>SMTIRSYKNLNLVRANIETESRQFIENKNYSIQSIGPMPGSRAGLRVVFTRPGVNLATVDIFYNGDGSTTIQYLTGANRSLGQELADHLFETINPAEFEQVNMVLQGFVETSVLPVLELSADESHIEFREHSRNAHTVVWKIISTSYQDELTVSLHITTGKLQIQGRPLSCYRVFTFNLAALLDLQGLEKVLIRQEDGKANIVQQEVARTYLQTVMADAYPHLHVTAEKLLVSGLCVKLAAPDLPDYCMLLYPELRTIEGVLKSKMSGLGMPVQQPAGFGTYFDKPAAHYILKPQFAATLRPEQ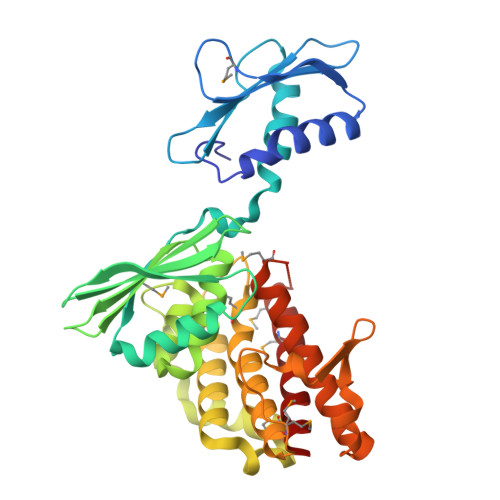INIISTAYTFFNVERHSLFHMETVVDASRMISDMARLMGKATRAWGIIKDLYIV[2x]>XMFIVNTNVPRASVPDGFLSELTQQLAQATGKPPQYIAVHVVPDQLMAFGGSSEPCALCSLHSIGKIGGAQNRSYSKLLCGLLAERLRISPDRVYINYYDMNAANVGWNNSTFA[6x]

Macrophage migration inhibitory factor (MIF) is expressed at high levels in various inflammatory diseases and cancer. Macrophage migration inhibitory factor promotes directional cell migration (or chemotaxis) of various cell types 2, 3, 4. Unlike canonical cytokines and chemokines, a trimeric MIF molecule has three tautomerase active sites at the trimer interfaces 23. Although the enzymatic activity is vestigial, there is accumulating evidence that the active site is important for receptor binding 24, 25.

To structurally verify the proposal for the inhibition of p110γ and p101 expression, we co‐crystallized 1, 2 and 12 with MIF. 12 is covalently bound to Pro1 in the middle of its structure and as a result occupies more of the pocket compared to 1 and 2. Because of this higher occupancy of the active site, 12 may stabilize better the conformation of the active site than 1 and 2, resulting in no disruption of MIF interactions with its receptor. In crystal packing, MIF:12 complexes revealed two trimers in a repeating three‐dimensional unit (or asymmetric unit), so each MIF trimer structure was analysed. The phenol ring of Tyr36 was moved from the original position (magenta) as shown in 1‐bound structure to a slightly open position (green) in 2‐bound structure, and to the fully open position (light pink) in 12‐bound structure. Apo‐MIF and MIF:12 complexes exhibit B‐factors under 5 Å2 for L2 loop, indicating low flexibility and possibly stable interactions with receptors. MIF:12 shows high B‐factors only for L1 and this also suggests that L1 may not be critical for receptor binding. 12 increased the flexibility of L1, whereas other inhibitors did not. Thus, it is likely that 12 disrupts L1 interaction with either CXCR2 or CXCR4 and is also responsible for the partial inhibition of p110γ expression. In contrast, 12 did not significantly inhibit neutrophil recruitment.> DDATADSRKTYTLTDYLKNTYRLKLYSLRWISDHEYLYKQENNILVFNAEYGNSSVFLENSTFDEFGHSINDYSISPDGQFILLEYNYVKQWRHSYTASYDIYDLNKRQLITEERIPNNTQWVTWSPVGHKLAYVWNNDIYVKIEPNLPSYRITWTGKEDIIYNGITDWVYEEEVFSAYSALWWSPNGTFLAYAQFNDTEVPLIEYSFYSDESLQYPKTVRVPYPKAGAVNPTVKFFVVNTDSLSSVTNATSIQITAPASMLIGDHYLCDVT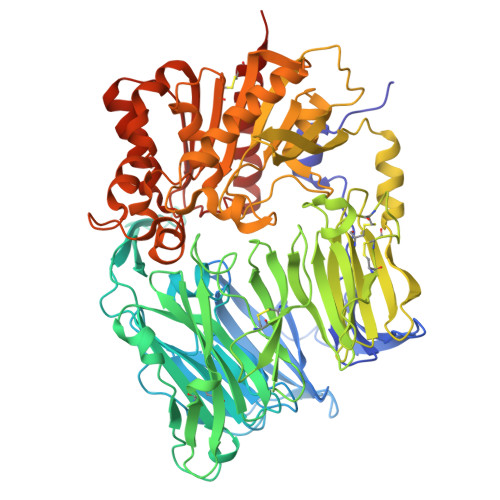WATQERISLQWLRRIQNYSVMDICDYDESSGRWNCLVARQHIEMSTTGWVGRFRPSEPHFTLDGNSFYKIISNEEGYRHICYFQIDKKDCTFITKGTWEVIGIEALTSDYLYYISNEYKGMPGGRNLYKIQLSDYTKVTCLSCELNPERCQYYSVSFSKEAKYYQLRCSGPGLPLYTLHSSVNDKGLRVLEDNSALDKMLQNVQMPSKKLDFIILNETKFWYQMILPPHFDKSKKYPLLLDVYAGPCSQKADTVFRLNWATYLASTENIIVASFDGRGSGYQGDKIMHAINRRLGTFEVEDQIEAARQFSKMGFVDNKRIAIWGWSYGGYVTSMVLGSGSGVFKCGIAVAPVSRWEYYDSVYTERYMGLPTPEDNLDHYRNSTVMSRAENFKQVEYLLIHGTADDNVHFQQSAQISKALVDVGVDFQAMWYTDEDHGIASSTAHQHIYTHMSHFIKQCFSLPHHHHHH> SNAADTVVQAGETVNGGTLTNHDNQIVLGTANGMTISTGLEYGPDNEANTGGQWIQNGGIANNTTVTGGGLQRVNAGGSVSDTVISAGGGQSLQGQAVNTTLNGGEQWVHEGGIATGTVINEKGWQAVKSGAMATDTVVNTGAEGGPDAENGDTGQTVYGDAVRTTINKNGRQIVAAEGTANTTVVYAGGDQTVHGHALDTTLNGGYQYVHNGGTASDTVVNSDGWQIIKEGGLADFTTVNQKGKLQVNAGGTATNVTLTQGGALVTSTAATVTGSNRLGNFTVENGNADGVVLESGGRLDVLEGHSAWKTLVDDGGTLAVSAGGKATDVTMTSGGALIADSGATVEGTNASGKFSIDGISGQASGLLLENGGSFTVNAGGLASNTTVGHRGTLTLAAGGSLSGRTQLSKGASMVLNGDVVSTGDIVNAGEIRFDNQTTPDAALSRAVAKGDSPVTFHKLTTSNLTGQGGTINMRVRLDGSNASDQLVINGGQATGKTWLAFTNVGNSNLGVATSGQGIRVVDAQNGATTEEGAFALSRPLQAGAFNYTLNRDSDEDWYLRSEN

The best-characterised SAAT, antigen 43 (Ag43), is a protein that contributes to cell aggregation and biofilm formation in commensal Escherichia coli K-12 as well as in major pathotypes including enterohemorrhagic E. coli (EHEC) and uropathogenic E. coli (UPEC). Ag43 possesses a modular domain organisation that is common throughout the ATs, which encompasses an N-terminal signal sequence that directs the secretion of the protein across the inner membrane, a passenger (α) domain that is responsible for the function of the protein, and a C-terminal translocator (β) domain that facilitates the translocation of the functional α-domain to the cell surface. After translocation, the Ag43 α-domain (α43) is cleaved but remains attached to the cell via non-covalent interactions. Similar to α43a 13, the α-domain of all three Ag43 variants folds into an L-shaped right-handed three-stranded β-helix, with each turn of the β-spine comprising three β-strands linked by loop regions.

The α43_UTI89 and α43_EDL933 structures in this work correspond to the uncleaved α-domains. To investigate whether this mechanism of self-association is conserved in Ag43UTI89, which imparts a reduced aggregation phenotype, we first examined its oligomerisation in the crystal lattice. Generation of crystallographically related molecules of α43_UTI89 (i.e. symmetrically related molecules in the crystal lattice) revealed a head-to-tail dimer repeated along the crystal, which resembled the α43a–α43a functional dimer. However, while α43a trans-dimers are stabilised by two interfaces consisting of a total of 18 hydrogen bonds and two salt bridges, α43_UTI89 dimers are formed via interactions from a single interface comprising 13 hydrogen bonds. To test if this α43_UTI89 crystallographic interface was indeed involved in mediating bacterial aggregation, we constructed a mutant with seven amino acid substitutions (Ag43UTI89-mt: T32G, N60G, D79G, T80G, T98G, N100G, N137G; mutations to glycine were adopted as glycine residues are enriched in the loop regions of Ag43 β-helices; Supplementary Fig. 2). Modification of the single interface in Ag43UTI89 completely abolished the ability of this protein to promote aggregation, confirming the self-association interface observed in the crystal lattice. Conversely, the reduced aggregation phenotype of Ag43UTI89 is a direct result of the weaker α43_UTI89 dimers, which are only stabilised by a single interface encompassing 13 hydrogen bonds. It appears that the inability of α43_UTI89 to form a double interface may be due to the presence of long sidechains on residues such as R161 or D133 in the F2–F3 loops mapping in the lower part of the β-helix, which in a head-to-tail association via a double interface would result in steric clashes between interacting proteins, although we cannot rule out other amino acids that might also interfere with this interaction.>SNAMAGPSDRTFSDQTEEIMQATYRALREHGYADLTIQRIADEYGKSTAAVHYYYDTKDDLLAAFLDYLLERFVDSIHDVETTDPEARLNLLLDELLVKPQENPDLSVALLEMRSQAPYKEAFSDRFRQNDEYVRYMLKAVINHGIDEGVFTDVDAEHVTRSLLTIIDGARTR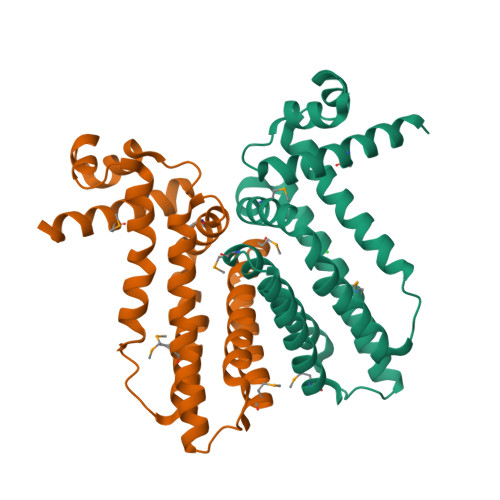AVMLDDTEELETARQTASEYADAMLQ[4x]> SNAMTIQHQFAENLSRLKKEHGLKNHQIAELLNVQTRTVAYYMSGETKPDIEKLIRLATYF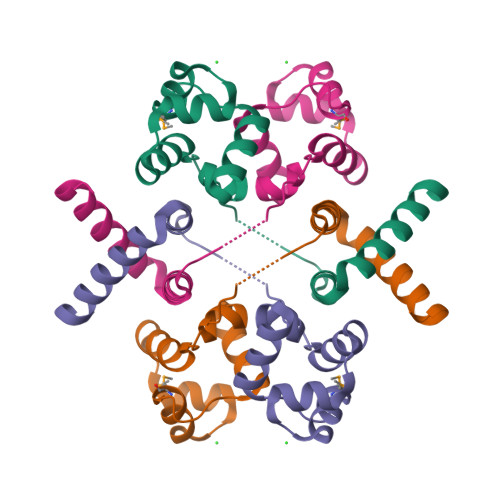HLSIDELVGYVQEDKVWNDLSLKQWLLSLNLRSEEEIAKIKILVDTVETLYPN>[2x]GPLGSPEFQKTKPFSVPNLPLNTLSNSRVPSLINAMMISRDHGQMVQFQNGRVTLDGQLQGTTPTSLSQLCKIRGKVFHASGGNGLNLTELDGSA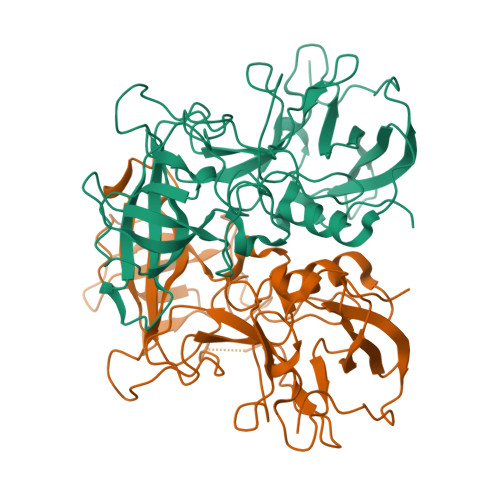YHAFESPAPIGFPDIGDCDWHMSATATNNFTGSSNEYQILIKQESAFAPHLGHVQADNLSAGANTDLIVSLSWISPVSDQHRHDVDPWVIPRYGSSLTEAAQLAPPIYPPGFGEAIVFFMSDFPVVSGVNGMRIPCTLPQEYVAHFVNEQAPTRGEAALLHYVDPDTHRNLGEFKMYPEGFMTCVPNSSGSGPQTLPINGVFTFVSWVSRFYQLKPVGTAGPARRLGIRRS> AGTKLSLMPWFHGKITREQAERLLYPPETGLFLVREST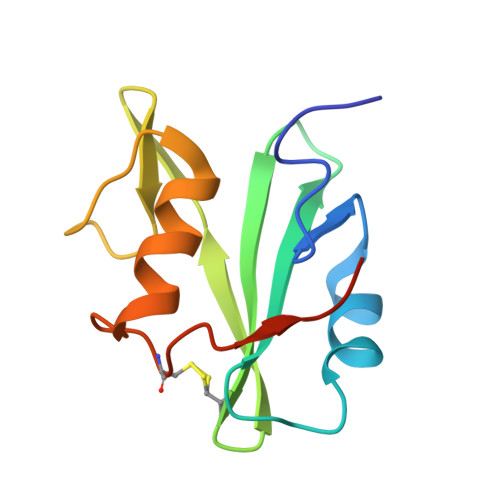NYPGDYTLCVSCDGKVEHYRIMYHASKLSIDEEVYFENLMQLVEHYTSDADGLCTRLIKPKVMEGTVA> AKLGAVYTEGGFVEGVNKKLGLLGDSVDIFKGIPFAAPTKALENPQPHPGWQGTLKAKNFKKRCLQATITQDSTYGDEDCLYLNIWVPQGRKQVSRDLPVMIWIYGGAFLMGSGHGANFLNNYLYDGEEIATRGNVIVVTFNYRVGPLGFLSTGDANLPGNYGLRDQHMAIAWVKRNIAAFGGDPNNITLFGESAGGASVSLQTLSPYNKGLIRRAISQSGVALSPWVIQKNPLFWAKKVAEKVGCPVGDAARMAQCLKVTDPRALTLAYKVPLAGLEYPMLHYVGFVPVIDGDFIPADPINLYANAADIDYIAGTNNMDGHIFASIDMPRINKGNKKVTEEDFYKLVSEFTITKGLRGAKTTFDVYTESWAQDPSQEN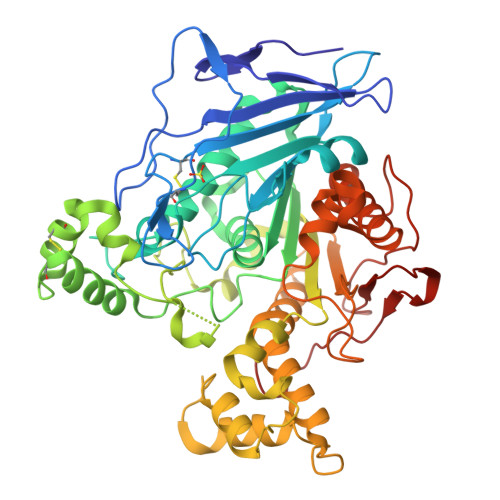KKKTVVDFETDVLFLVPTEIALAQHRANAKSAKTYAYLFSHPSRMPVYPKWVGADHADDIQYVFGKPFATPTGYRPQDRTVSKAMIAYWTNFAKTGDPNMGDSAVPTHWEPYTTENSGYLEITKKMGSSSMKRSLRTNFPGIH>MGLPRGSFFWLLLLLTAACSGLLFALYFSAVQRYP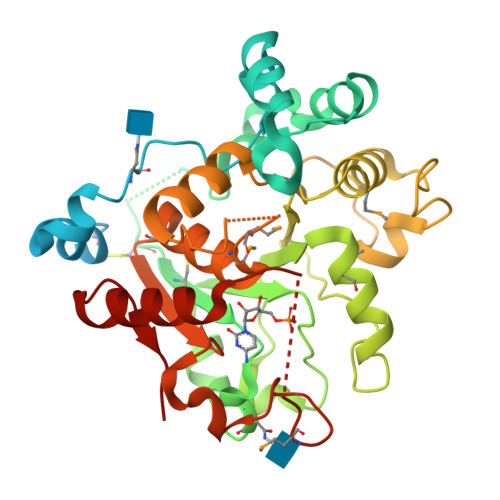GPAAGARDTTSFEAFFQSKASNSWTGKGQACRHLLHLAIQRHPHFRGLFNLSIPVLLWGDLFTPALWDRLSQHKAPYGWRGLSHQVIASTLSLLNGSESAKLFAPPRDTPPKCIRCAVVGNGGILNGSRQGPNIDAHDYVFRLNGAVIKGFERDVGTKTSFYGFTVNTMKNSLVSYWNLGFTSVPQGQDLQYIFIPSDIRDYVMLRSAILGVPVPEGLDKGDRPHAYFGPEASASKFKLLHPDFISYLTERFLKSKLINTHFGDLYMPSTGALMLLTALHTCDQVSAYGFITSNYWKFSDHYFERKMKPLIFYANHDLSLEAALWRDLHKAGILQLYQR[6x]>[2x]GPMVTGGGAAPPGTVTEPLPSVIVLSAGRKMAAAAAAASGPGCSSAAGAGAAGVSEWLVLRDGCMHCDADGLHSLSYHPALNAILAVTSRGTIKVIDGTSGATLQASALSAKPGGQVKCQYISAVDKVIFVDDYAVGCRKDLNGILLLDTALQTPVSKQDDVVQLELPVTEAQQLLSACLEKVDISSTEGYDLFITQLKDGLKNTSHETAANHKVAKWATVTFHLPHHVLKSIASAIVNELKKINQNVAALPVASSVMDRLSYLLPSARPELGVGPGRSVDRSLMYSEANRRETFTSWPHVGYRWAQPDPMAQAGFYHQPASSGDDRAMCFTCSVCLVCWEPTDEPWSEHERHSPNCPFVKGEHTQNVPLSVTLATSPAQFPCTDGTDRISCFGSGSCPHFLAAATKRGKICIWDVSKLMKVHLKFEINAYDPAIVQQLILSGDPSSGVDSRRPTLAWLEDSSSCSDIPKLEGDSDDLLEDSDSEEHSRSDSVTGHTSQKEAMEVSLDITALSILQQPEKLQWEIVANVLEDTVKDLEELGANPCLTNSKSEKTKEKHQEQHNIPFPCLLAGGLLTYKSPATSPISSNSHRSLDGLSRTQGESISEQGSTDNESCTNSELNSPLVRRTLPVLLLYSIKESDEKAGKIFSQMNNIMSKSLHDDGFTVPQIIEMELDSQEQLLLQDPPVTYIQQFADAAANLTSPDSEKWNSVFPKPGTLVQCLRLPKFAEEENLCIDSITPCADGIHLLVGLRTCPVESLSAINQVEALNNLNKLNSALCNRRKGELESNLAVVNGANISVIQHESPADVQTPLIIQPEQRNVSGGYLVLYKMNYATRIVTLEEEPIKIQHIKDPQDTITSLILLPPDILDNREDDCEEPIEDMQLTSKNGFEREKTSDISTLGHLVITTQGGYVKILDLSNFEILAKVEPPKKEGTEEQDTFVSVIYCSGTDRLCACTKGGELHFLQIGGTCDDIDEADILVDGSLSKGIEPSSEGSKPLSNPSSPGISGVDLLVDQPFTLEILTSLVELTRFETLTPRFSATVPPCWVEVQQEQQQRRHPQHLHQQHHGDAAQHTRTWKLQTDSNSWDEHVFELVLPKACMVGHVDFKFVLNSNITNIPQIQVTLLKNKAPGLGKVNALNIEVEQNGKPSLVDLNEEMQHMDVEESQCLRLCPFLEDHKEDILCGPVWLASGLDLSGHAGMLTLTSPKLVKGMAGGKYRSFLIHVKAVNERGTEEICNGGMRPVVRLPSLKHQSNKGYSLASLLAKVAAGKEKSSNVKNENTSGTRKSENLRGCDLLQEVSVTIRRFKKTSISKERVQRCAMLQFSEFHEKLLNTLCRKTDDGQITEHAQSLVLDTLCWLAGVHSNGPGSSKEGNENLLSKTRKFLSDIVRVCFFEAGRSIAHKCARFLALCISNGKCDPCQPAFGPVLLKALLDNMSFLPAATTGGSVYWYFVLLNYVKDEDLAGCSTACASLLTAVSRQLQDRLTPMEALLQTRYGLYSSPFDPVLFDLEMSGSSCKNVYNSSIGVQSDEIDLSDVLSGNGKVSSCTAAEGSFTSLTGLLEVEPLHFTCVSTSDGTRIERDDAMSSFGVTPAVGGLSSGTVGEASTALSSAAQVALQSLSHAMASAEQQLQVLQEKQQQLLKLQQQKAKLEAKLHQTTAAAAAAASAVGPVHNSVPSNPVAAPGFFIHPSDVIPPTPKTTPLFMTPPLTPPNEAVSVVINAELAQLFPGSVIDPPAVNLAAHNKNSNKSRMNPLGSGLALAISHASHFLQPPPHQSIIIERMHSGARRFVTLDFGRPILLTDVLIPTCGDLASLSIDIWTLGEEVDGRRLVVATDISTHSLILHDLIPPPVCRFMKITVIGRYGSTNARAKIPLGFYYGHTYILPWESELKLMHDPLKGEGESANQPEIDQHLAMMVALQEDIQCRYNLACHRLETLLQSIDLPPLNSANNAQYFLRKPDKAVEEDSRVFSAYQDCIQLQLQLNLAHNAVQRLKVALGASRKMLSETSNPEDLIQTSSTEQLRTIIRYLLDTLLSLLHASNGHSVPAVLQSTFHAQACEELFKHLCISGTPKIRLHTGLLLVQLCGGERWWGQFLSNVLQELYNSEQLLIFPQDRVFMLLSCIGQRSLSNSGVLESLLNLLDNLLSPLQPQLPMHRRTEGVLDIPMISWVVMLVSRLLDYVATVEDEAAAAKKPLNGNQWSFINNNLHTQSLNRSSKGSSSLDRLYSRKIRKQLVHHKQQLNLLKAKQKALVEQMEKEKIQSNKGSSYKLLVEQAKLKQATSKHFKDLIRLRRTAEWSRSNLDTEVTTAKESPEIEPLPFTLAHERCISVVQKLVLFLLSMDFTCHADLLLFVCKVLARIANATRPTIHLCEIVNEPQLERLLLLLVGTDFNRGDISWGGAWAQYSLTCMLQDILAGELLAPVAAEAMEEGTVGDDVGATAGDSDDSLQQSSVQLLETIDEPLTHDITGAPPLSSLEKDKEIDLELLQDLMEVDIDPLDIDLEKDPLAAKVFKPISSTWYDYWGADYGTYNYNPYIGGLGIPVAKPPANTEKNGSQTVSVSVSQALDARLEVGLEQQAELMLKMMSTLEADSILQALTNTSPTLSQSPTGTDDSLLGGLQAANQTSQLIIQLSSVPMLNVCFNKLFSMLQVHHVQLESLLQLWLTLSLNSSSTGNKENGADIFLYNANRIPVISLNQASITSFLTVL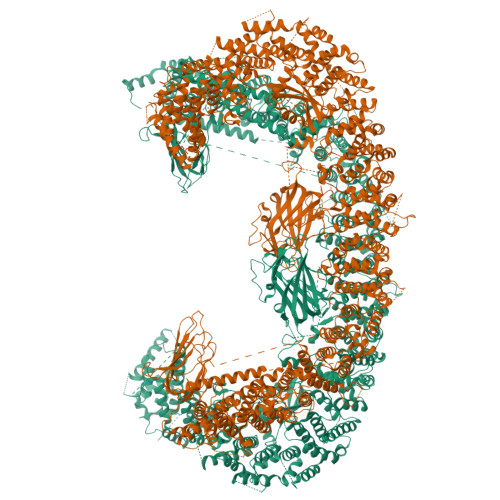AWYPNTLLRTWCLVLHSLTLMTNMQLNSGSSSAIGTQESTAHLLVSDPNLIHVLVKFLSGTSPHGTNQHSPQVGPTATQAMQEFLTRLQVHLSSTCPQIFSEFLLKLIHILSTERGAFQTGQGPLDAQVKLLEFTLEQNFEVVSVSTISAVIESVTFLVHHYITCSDKVMSRSGSDSSVGARACFGGLFANLIRPGDAKAVCGEMTRDQLMFDLLKLVNILVQLPLSGNREYSARVSVTTNTTDSVSDEEKVSGGKDGNGSSTSVQGSPAYVADLVLANQQIMSQILSALGLCNSSAMAMIIGASGLHLTKHENFHGGLDAISVGDGLFTILTTLSKKASTVHMMLQPILTYMACGYMGRQGSLATCQLSEPLLWFILRVLDTSDALKAFHDMGGVQLICNNMVTSTRAIVNTARSMVSTIMKFLDSGPNKAVDSTLKTRILASEPDNAEGIHNFAPLGTITSSSPTAQPAEVLLQATPPHRRARSAAWSYIFLPEEAWCDLTIHLPAAVLLKEIHIQPHLASLATCPSSVSVEVSADGVNMLPLSTPVVTSGLTYIKIQLVKAEVASAVCLRLHRPRDASTLGLSQIKLLGLTAFGTTSSATVNNPFLPSEDQVSKTSIGWLRLLHHCLTHISDLEGMMASAAAPTANLLQTCAALLMSPYCGMHSPNIEVVLVKIGLQSTRIGLKLIDILLRNCAASGSDPTDLNSPLLFGRLNGLSSDSTIDILYQLGTTQDPGTKDRIQALLKWVSDSARVAAMKRSGRMNYMCPNSSTVEYGLLMPSPSHLHCVAAILWHSYELLVEYDLPALLDQELFELLFNWSMSLPCNMVLKKAVDSLLCSMCHVHPNYFSLLMGWMGITPPPVQCHHRLSMTDDSKKQDLSSSLTDDSKNAQAPLALTESHLATLASSSQSPEAIKQLLDSGLPSLLVRSLASFCFSHISSSESIAQSIDISQDKLRRHHVPQQCNKMPITADLVAPILRFLTEVGNSHIMKDWLGGSEVNPLWTALLFLLCHSGSTSGSHNLGAQQTSARSASLSSAATTGLTTQQRTAIENATVAFFLQCISCHPNNQKLMAQVLCELFQTSPQRGNLPTSGNISGFIRRLFLQLMLEDEKVTMFLQSPCPLYKGRINATSHVIQHPMYGAGHKFRTLHLPVSTTLSDVLDRVSDTPSITAKLISEQKDDKEKKNHEEKEKVKAENGFQDNYSVVVASGLKSQSKRAVSATPPRPPSRRGRTIPDKIGSTSGAEAANKIITVPVFHLFHKLLAGQPLPAEMTLAQLLTLLYDRKLPQGYRSIDLTVKLGSRVITDPSLSKTDSYKRLHPEKDHGDLLASCPEDEALTPGDECMDGILDESLLETCPIQSPLQVFAGMGGLALIAERLPMLYPEVIQQVSAPVVTSTTQEKPKDSDQFEWVTIEQSGELVYEAPETVAAEPPPIKSAVQTMSPIPAHSLAAFGLFLRLPGYAEVLLKERKHAQCLLRLVLGVTDDGEGSHILQSPSANVLPTLPFHVLRSLFSTTPLTTDDGVLLRRMALEIGALHLILVCLSALSHHSPRVPNSSVNQTEPQVSSSHNPTSTEEQQLYWAKGTGFGTGSTASGWDVEQALTKQRLEEEHVTCLLQVLASYINPVSSAVNGEAQSSHETRGQNSNALPSVLLELLSQSCLIPAMSSYLRNDSVLDMARHVPLYRALLELLRAIASCAAMVPLLLPLSTENGEEEEEQSECQTSVGTLLAKMKTCVDTYTNRLRSKRENVKTGVKPDASDQEPEGLTLLVPDIQKTAEIVYAATTSLRQANQEKKLGEYSKKAAMKPKPLSVLKSLEEKYVAVMKKLQFDTFEMVSEDEDGKLGFKVNYHYMSQVKNANDANSAARARRLAQEAVTLSTSLPLSSSSSVFVRCDEERLDIMKVLITGPADTPYANGCFEFDVYFPQDYPSSPPLVNLETTGGHSVRFNPNLYNDGKVCLSILNTWHGRPEEKWNPQTSSFLQVLVSVQSLILVAEPYFNEPGYERSRGTPSGTQSSREYDGNIRQATVKWAMLEQIRNPSPCFKEVIHKHFYLKRVEIMAQCEEWIADIQQYSSDKRVGRTMSHHAAALKRHTAQLREELLKLPCPEGLDPDTDDAPEVCRATTGAEETLMHDQVKPSSSKELPSDFQL> MEDIEKIKPYVRSFSKALDELKPEIEKLTSKSLDEQLLLLSDERAKLELINRYAYVLSSLMFANMKVLGVKDMSPILGELKRVKSYMDKAKQYDNRITKSNEKSQAEQEKAKNIISNVLDGNKNQFEPSISRSNFQGKHTKFENDELAESTTTKIIDSTDHIRKASSKKSKRLDKVGK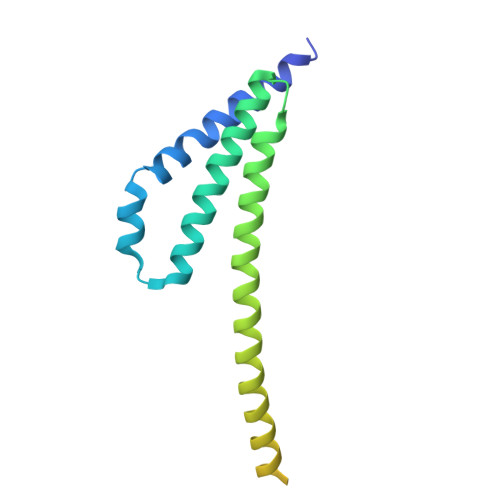KKGGKK DotI is a 23 kDa inner membrane protein essential for intracellular growth of L. pneumophila within mammalian and protozoan cells. DotI has one transmembrane domain in its N-terminal region, followed by a periplasmic domain13. DotI is conserved in all of the identified type IVB secretion systems, including the conjugation systems of R64 and related plasmids. Structural analysis of the periplasmic domains of DotI and its R64 ortholog TraM demonstrated that DotI and TraM are structural homologs of the T4ASS protein VirB8.

DotIC crystallized in two distinct forms (Form I and Form II) under different conditions. The structure model of Form I (space group: P21212) was refined to a resolution of 2.2 Å with the working R and the free R factor of 19.1% and 23.5%, respectively, and Form II (space group: I432) to a resolution of 3.5 Å with the working R and the free R factor of 17.9% and 21.6%, respectively. Form I and Form II contain eight and four molecules in its asymmetric unit, respectively, and the structures of these molecules are almost identical. DotIC is a single domain protein composed of four helices (α1 - α4) in one half and one β-sheet in the other half. The octameric rings are also present in the Form II crystal. The four molecules in the asymmetric unit of Form II are arranged as a stack of a quarter of the ring, and the crystallographic four-fold axis produces a stack of two octameric rings. The oligomerization of DotIC is also observed in solution. Although DotIC is in a monomeric state during purification, an oligomeric peak appears in size exclusion chromatography under the crystallization condition. SEC-MALS measurement showed that the apparent molecular weight of the oligomer is 263 kDa, which is consistent with the molecular weight of the stack of two octameric rings. This evidence suggests that octameric ring formation is not a crystal packing artifact, but instead an intrinsic property of the DotIC molecule.

>GSHMQSDSAVLQWANQAAIAAFTYNFVNYRDELQASSGFFTAEGWDQFLGALEQSNNLDAVKAKKLVVSAVATRAPIILQKGVLNGRYSWRVQMPILVTYQSASEFTQQNNVVTMLITRVSTLNSPRGIGISQFVVGPASGGVS[4x]> TVASISSGPKHTQKVPILTANETGATMPVLPSDSIETRTTYMHFNGSETDVECFLGRAACVHVTEIQNKDATGIDNHREAKLFNDWKINLSSLVQLRKKLELFTYVRFDSEYTILATASQPDSANYSSNLVVQAMYVPPGAPNPKEWDDYTWQSASNPSVFFKVGDTSRFSVPYVGLASAYNCFYDGYSHDDAETQYGITVLNHMGSMAFRIVNEHDEHKTLVKIRVYHRAKHVEAWIPRAPRALPYTSIGRTNYPKNTEPVIKKRKGDIKSY;> SPNVEACGYSDRVQQITLGNSTITTQEAANAVVCYAEWPEYLPDVDASDVNKTSKPDTSVCRFYTLDSKTWTTGSKGWCWKLPDALKDMGVFGQNMFFHSLGRSGYTVHVQCNATKFHSGCLLVVVIPEHQLASHEGGNVSVKYTFTHPGERGIDLS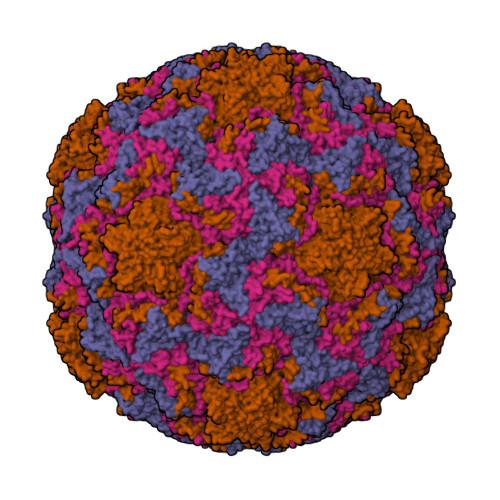SANEVGGPVKDVIYNMNGTLLGNLLIFPHQFINLRTNNTATIVIPYINSVPIDSMTRHNNVSLMVIPIAPLTVPTGATPSLPITVTIAPMCTEFSGIRSKSIVPQ;> GLPTTTLPGSGQFLTTDDRQSPSALPNYEPTPRIHIPGKVHNLLEIIQVDTLIPMNNTHTKDEVNSYLIPLNANRQNEQVFGTNLFIGDGVFKTTLLGEIVQYYTHWSGSLRFSLMYTGPALSSAKLILAYTPPGARGPQDRREAMLGTHVVWDIGLQSTIVMTIPWTSGVQFRYTDPDTYTSAGFLSCWYQTSLILPPETTGQVYLLSFISACPDFKLRLMKDTQTISQTVALTE;> GAQVSTQKSGSHENQNILTNGSNQTFTVINYYKDAASTSSAGQSLSMDPSKFTEPVKDLMLKGAPALN>[6x]KLFITEGYEVGRVNGLAVIGESAGIVLPIIAEVTPSMSKSEGRVIATGRLQEIAREAVMNVSAIIKKYTGRDISNMDVHIQF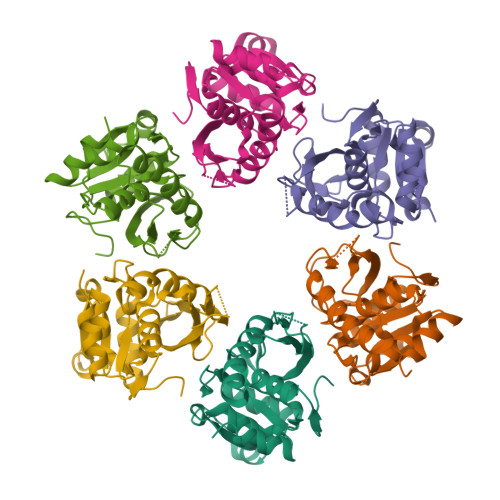VGTYEGVEGDSASISIATAVISAIEGIPVDQSVAMTGSLSVKGEVLPVGGVTQKIEAAIQAGLKKVIIPKDNIDDVLLDAEHEGKIEVIPVSRINEVLEHVLEDGKKKNRLMSKFKELELAAV{1-[(2,5-dimethylphenyl)methyl]-1H-benzimidazol-2-yl}methanol | C17 H18 N2 O | 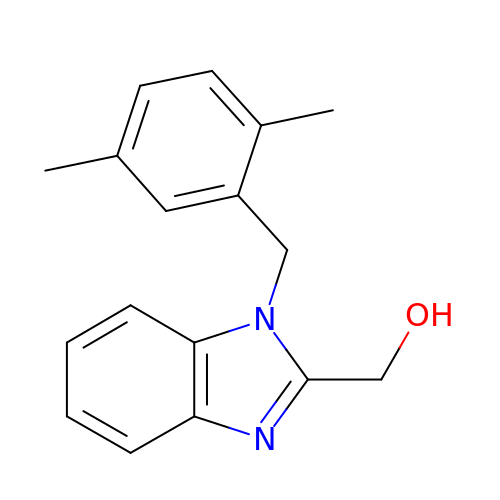RZRPPZWEPMDGEI-UHFFFAOYSA-N>MQRGKV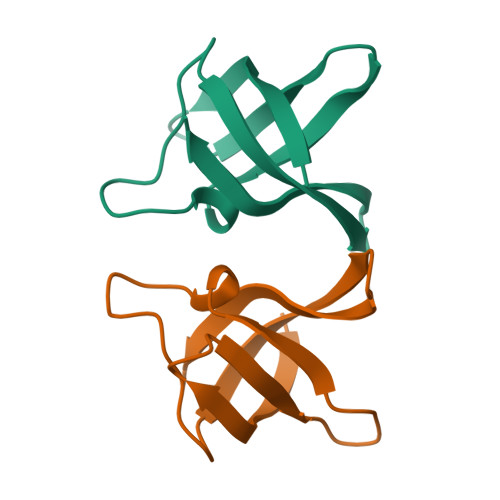KWFNNEKGYGFIEVEGGSDVFVHFTAIQGEGFKTLEEGQAVSFEIVQGNRGPQAANVVKL[2x]>[4x]MNDNVAWFKQAKYGMMIHWGLYSLLAGEYRGESSSAYAEWIQSKFQIPNAEYGNLATAFNPLYFDAKKIVALAKQCGMQYLVVTTKHHDGFAMYHSKVDAYNVYDATPFHRDIIGELAEACQKAGLKFGLYYSQDLDWHDPNGGGYKSNDVETAGTTWDNSWDFPDEDQKNFDLCFDNKILPQIKEIMSNYGDIATAWFDVPMTLSEAQSQTIYDTVRELQPNCLINSRLGNGKYDFVSLGDNEIPKNKEDMNKTDVDYNEITGFKPSPLGLYATAGTINDSWGFSYHDQNWKTPRTLYRYKQHLNDFGINYLLNVGLDPLGRVPMMAEENLLAAKALEDEANRL

Lactobacillus casei produces a GH29A α-fucosidase, AlfC, that is ~104-fold more active on α(1-6)-fucosyl linkages compared to other linkages. This enzyme is particularly relevant because α(1-6) linkages form the basis of human core fucosylation, which significantly impacts the function of glycoproteins such as antibodies. AlfC is a single-domain enzyme that adopts a (β/α)8 fold typical of GH29 enzymes, with an active site at the center of the barrel. Our results suggest that AlfC employs a conserved hydrolytic mechanism with a specific subsite that accommodates GlcNAc in α(1,6)-linkages, while AlfC tranfucosidase mutants work by shifting equilibrium between open and closed conformations of an active-site loop.

The mutation of a glutamic acid residue at position 274 to alanine (AlfCE274A) has been shown to convert AlfC from a hydrolase into an efficient transfucosidase that can transfer a fucose moiety to an acceptor (e.g., N-acetylglucosamine [GlcNAc]) from a simple fucosyl donor (e.g., α-fucosyl fluoride) with nearly quantitative yields. We solved the X-ray crystal structures of both of these enzymes. They exhibited no major conformational changes compared to AlfCWT, with CαRMSD < 0.25 Å for each of the enzymes. Only AlfCE274A showed a subtle change near the site of mutation, with a displacement of the W198 side chain ~4 Å due to an alternate rotamer conformation in order to occupy the cavity left by E274A. The point mutant AlfCE274A is markedly more dynamic and solvent accessible, particularly in the regions surrounding R229 and D242. These residues interact to mediate open and closed conformations in MD simulations, with these results consistent with AlfCE274A sampling more open conformations. The marked perturbation in R229 provides a potential rationale for the azide rescue seen with AlfCE274A, if azide ions occupy the E274A cavity to stabilize R229 and promote closed conformations. The reaction, monitored by 19F NMR, revealed that only E274A could be rescued by the addition of azide, reaching a reaction speed of about one-third of the wild-type speed. The HDX-MS analysis suggests that AlfCE274A and AlfCN243A are transfucosidase mutants that work by shifting the dynamic equilibrium of AlfC toward a more open conformation.> GMDELELRIRKAEKLVQDAKKEFEMGLYERCCSTAYYAMFHAAKAMLLGYGRDSKTHRGTIYLIWECREELGLSDDDCSKLSRAFDL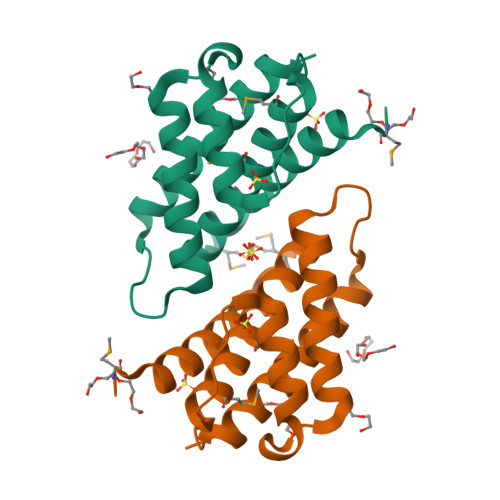REESDYGIYKEVSKDLAIKILKDAEIFVQKAKNAVNKNR> GGAGC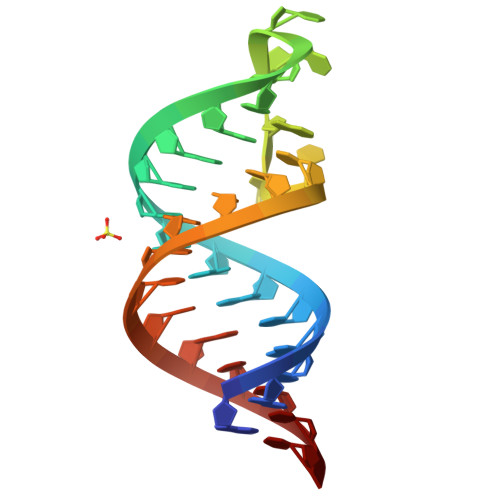GGGCGGGUUCGAGUCCCGUCCGUUCC>FKEQSFVYKKDGNFLKLPDTDCRQTPPFLVLLVTSSHKQLAERMAIRQTWGKERMVKGKQLKTFFLLGTTSSAAETKEVDQESQRHGDIIQKDFLDVYYNLTLKTMMGIEWVHRFCPQAAFVMKTDSDMFINVDYLTELLLKKNRTTRFFTGFLKLNEFPIRQPFSKWFVSKSEYPWDRYPPFCSGTGYVFSGDVASQVYNVSKSVPYIKLEDVFVGLCLERLNIRLEELHSQPTFFPGGLRFSVCLFRRIVACHFIKPRTLLDYWQALENSRGEDCP[2x]

Human β1,3-galactosyltransferase 5 (β3GalT5) is a key enzyme involved in the synthesis of glycans on glycoproteins and glycolipids that are associated with various important biological functions, especially tumor malignancy and cancer progression, and has been considered as a promising target for development of anticancer agents. The catalytic domain adopts a mixed α/β Rossmann-like fold commonly observed in the GT-A glycosyltransferases superfamily and consists of a seven-stranded β sheet core (β1, β2, β3, β4, β5, β6, and β7) surrounded primarily by α helices (α1, α2, α3, α4, α5, α6, and α7), a two-strand antiparallel β sheet (β5′ and β7’),23 and an additional 13-residue α helix (α8) at the C terminus. Based on the structures obtained from our experiments, β3GalT5 catalyzes the transfer of galactose from UDP-Gal to a broad spectrum of glycan acceptors with an SN2-like mechanism; however, in the absence of a glycan acceptor, UDP-Gal is slowly converted to UDP and two other products, one is galactose through an SN2-like mechanism with water as an acceptor and the other is an oxocarbenium-like product, presumably through an SN1-like mechanisms. While β3GalT5 selectively binds to UDP-Gal as the donor substrate, it exhibits broader selectivity for acceptor substrates.

In total, we obtained eight structures, including β3GalT5 in complex with UDP-Gal, Gb4 glycan, GlcNac-β1,3-Gal, GlcNAc-β1,3-GalNAc, and Man-β1,6-Man. All structures belong to the P1 21 1 space group, with each asymmetric unit containing two protein molecules. Using disaccharides as substrates and measuring the end point UDP concentration after 1 h reaction time, we have selected Man-β1,6-Man and GlcNAc-β1,3-GalNAc-α-Thr in addition to Gb4 glycan and GlcNAc-β1,3-Gal-OMe for further structural studies of the enzyme–substrate complex obtained from β3GalT5 cocrystallized with UDP-Gal and soaked with various acceptors. The acceptor binding moiety has relatively fewer interactions in comparison to the donor binding moiety, resulting in a wider tolerance to different acceptors. The indole lid is turned off when no receptor is bound but is activated by forming a stacking interaction with the nonreducing end of acceptor.> MIDADDYTVNLTSHTTLANIPSGAIIAVSESLTGKSVTSAGWVKADPTVFPEVTGDTGEAVIVYKHTGTASTSTLLSYHDSPTYQFV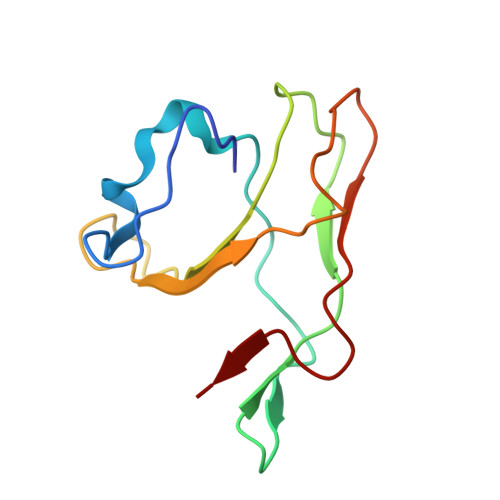IPNGSDIRVIWPTDGFIRF> MPQNVDKILDHAPLFREPEYQEMLAGKAKLENMPPADKVVEIADWTKSWEYREKNFARESLSVNPAKACQPLGAVFVASGFERTMSFVHGSQGCVAYYRSHLSRHFKEPSSAVSSSMTEDAAVFGGLNNMVDGLANTYKLYDPKMIAVSTTCMAEVIGDDL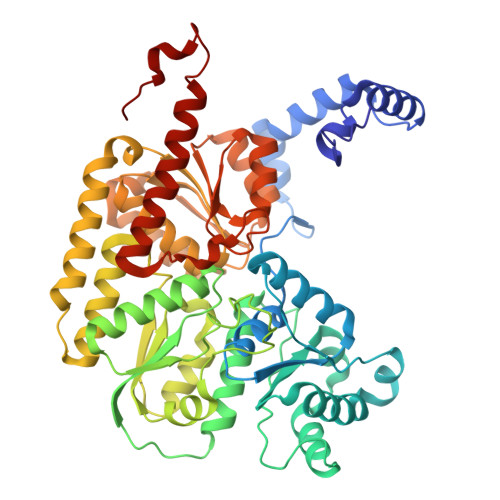HAFIQTAKGKGSVPEEFDVPFAHTPAFVGSHVTGYDNMLKGILEHFWKGRTPVPNRSVNIIPGFDGFAVGNNRELKRILGMMGVQYTILSDVSDQFDTPSDGEYRMYDGGTKIEAARDAVNADYTISLQEYCTPKTLEYCQSFGQKTASFHYPLGIGATDDLLQKLSEISGKPVPQELEMERGRLVDALADSQAYLHGKTYAIYGDPDFVYGMARFILETGGEPKHCLATNGSKAWEAQMQELFDSSPFGVGCKAWGGKDLWHMRSLLATEKVDLLIGNSYGKYLERDTDTPLIRLMFPIFDRHHHHRFPVWGYQGALRVLVTLLDKIFDKLDDDTIQAGVTDYSFDLTR2-HYDROXY BUTANE-1,4-DIOL 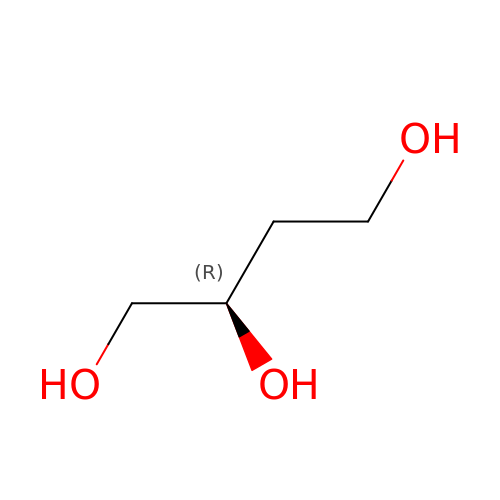| C4 H10 O3 | ARXKVVRQIIOZGF-SCSAIBSYSA-N> MKELIYIEEPSILFAHGQKCTDPRDGLALFGPLNQIYGIKSGVVGTQKGLQIFKSYLDKIQKPIYNHNNITRPMFPGFEAVFGCKWESQNIVFKEITDEEIRRYLFNASTHKRTYDLVTLFNDKIITANKNDEERVDVWFVIVPEEIYKYCRPNSVLPNELVQTKSLISKSKA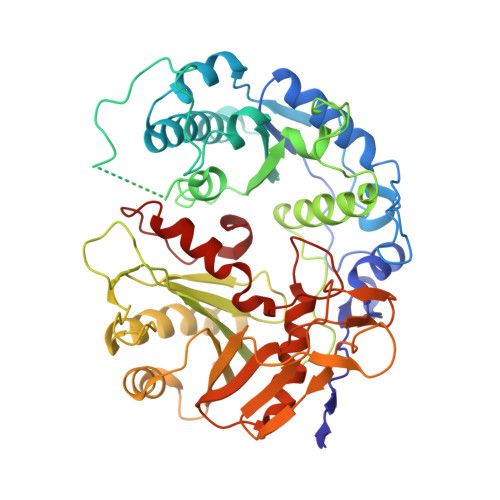KSFRYTPTLFEEFNKKLKEVEKEAKTYNYDAQFHDQLKARLLEHTIPTQILRESTLAWRDFKNTFGAPIRDFSKIEGHLAWTISTAAYYKAGGKPWKLGDIRPGVCYLGLVYKKIEKSKNPQNACCAAQMFLDNGDGTVFKGEVGPWYNPEKGEYHLKPKEAKALLTQALESYKEQNKSYPKEVFIHARTRFNDEEWNAFNEVTPKNTNLVGVTITKSKPLKLYKTEGAFPIMRGNAYIVDEKKAFLWTLGFVPKLQSTLSMEVPNPIFIEINKGEAEIQQVLKDILALTKLNYNACIYADGEPVTLRFANKIGEILTASTEIKTPPLAFKYYI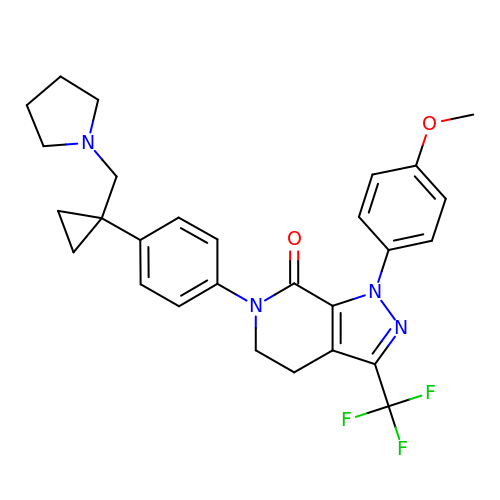1-(4-methoxyphenyl)-6-(4-(1-(pyrrolidin-1-ylmethyl)cyclopropyl)phenyl)-3-(trifluoromethyl)-5,6-dihydro-1H-pyrazolo[3,4-c]pyridin-7(4H)-one | C28 H29 F3 N4 O2 | VNHRSGCBTKUBAX-UHFFFAOYSA-N CEFOTAXIME, C3' cleaved, open, bound form | C14 H15 N5 O5 S2 | 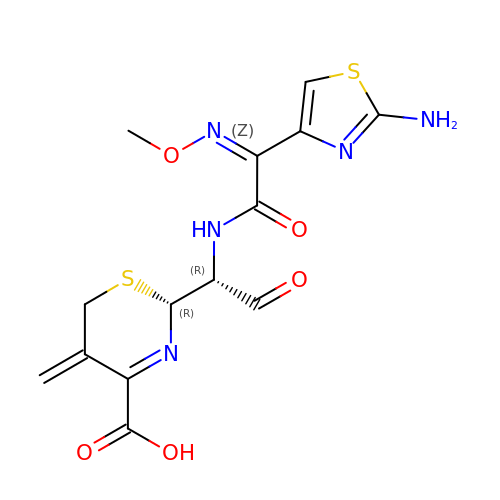NRYMPLKBKFIWQC-YVCCLBOHSA-N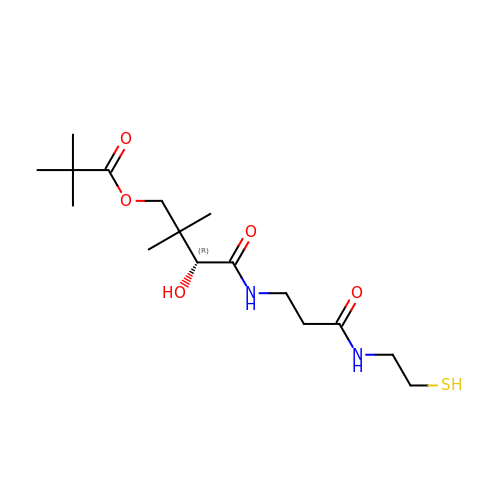(3R)-3-hydroxy-2,2-dimethyl-4-oxo-4-({3-oxo-3-[(2-sulfanylethyl)amino]propyl}amino)butyl 2,2-dimethylpropanoate | C16 H30 N2 O5 S | KVQSHCZSRKQWCB-LBPRGKRZSA-N>[2x]GAMDEKFIRETIETR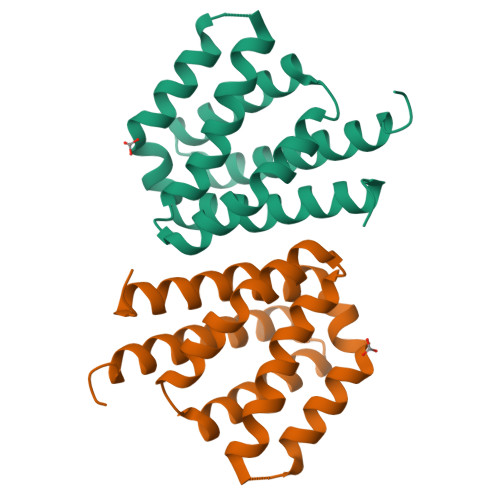IMMEVFCLENYFDKIAGSEELLEIKGEIDDVAASAAREIFDDSDERLHKLFIRASGNELIISLYEKIWDRIDLVRHLNERYVVSNREHKELIERIISGDKEGAIEKLKEHLKNVEAETIKNLYTY3-bromo-4-cyanobenzyl 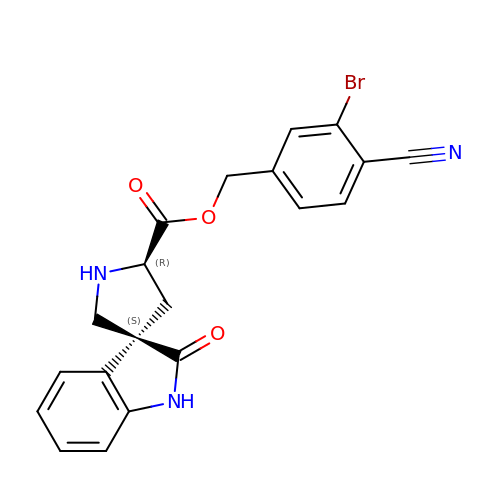(3S,5'R)-2-oxo-1,2-dihydrospiro[indole-3,3'-pyrrolidine]-5'-carboxylate | C20 H16 Br N3 O3 | DJYALAFSFGHFLN-YLJYHZDGSA-N>[2x]MKVLVVGSG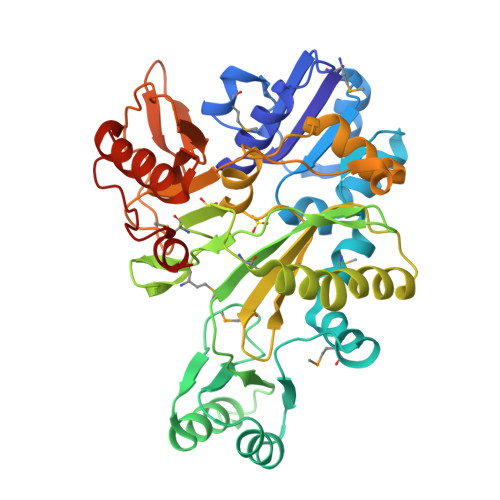GREHALLWKAAQSPRVKRLYAAPGNAGMEALAELVPWNGDVEALADWALAEGIDLTLVGPEAPLVEGIADAFQARGLLLFGPTQKAAMIEGSKAFAKGLMERYGIPTARYRVFREPLEALAYLEEVGVPVVVKDSGLAAGKGVTVAFDLHQAKQAVANILNRAEGGEVVVEEYLEGEEATVLALTDGETILPLLPSQDHKRLLDGDQGPMTGGMGAVAPYPMDEATLRRVEEEILGPLVRGLRAEGVVYRGVVYAGLMLTREGPKVLEFNARFGDPEAQALLPLLENDLVELALRVAEGRLAGTRLSWKEGAAACVVLAAPGYPESPRKGIPLHVPEPPEGVLVFHAGTRREGGRLVSAGGRVLNVVGLGRDLKEALERAYAYIPQVGFPGAVYRRDIGRRALARLST> MVRGGVATVGPSSLALAASALLGTLPQQTASHSGASLWVFGSRHLAAPAAAGGASNQDRTQPSAKPSAAEPELKLNFSLRPSVLSPLFPAWEQTRQINQRREHLMALLDAHQQLAEGLRITKDGVAASTDGADAGTTSSFAAGGVRAGVTRSARRRARNLQQVASQLRALLDATPGHPRGVTGLPTACPSPAHA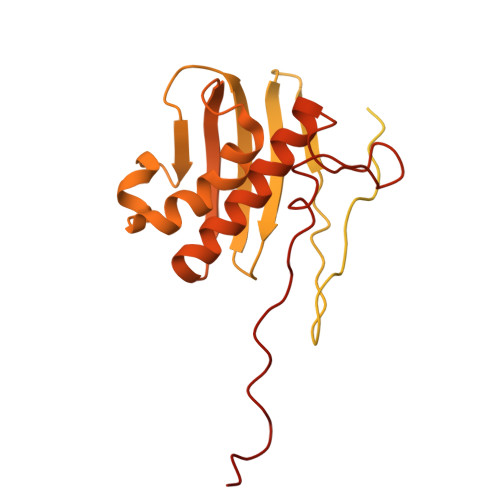VAYCGALEAALASPDAASTGARDFGAVARGDVSPWTHYAKHFAGRYAGAPQLQPLEVIYSRPDPAEVVRQLRRAAREQEALGISSSGGGSGEAGSGLAFPATSTSPEPAGPHIDLTGVTHARGKRKASAASVQLVPAGGAGITVNGVPLSSYFRDPACREKVLAPLALAGAETAYDVAARVKGGGMMGQAQAIATALARALCVQQPSLGATAGDGGNGEGPLAAMTRWDGRVVERQKPGQAGSRRGFQWVKR>[2x]GPLGSDSRQMTELLDSEQRQGLMIEQHVEAELANDPPNDLMWWRRLFRAIDKWAPPGQRLLLVTTEGRVIG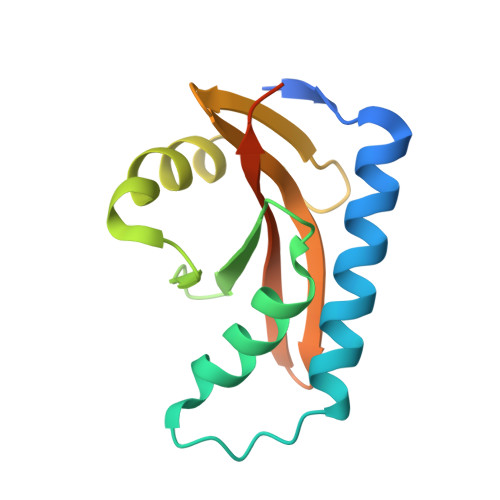AERSEMQIIRNFIGQADNADHPQKKKYGRVELVGPFSVRDGEDNYQLYLIRPASSSQSDFINLLFDR> MVLGKVVGTVVASRKEPRIEGLSLLLVRACDPDGTPTGGAVVCADAVGAGVGEVVLYASGSSARQTEVTNNRPVDATIMAIVDLVEMGGDVRFRKD;>MADALGMIEVRGFVGMVEAADAMVKAAKVELIGYEK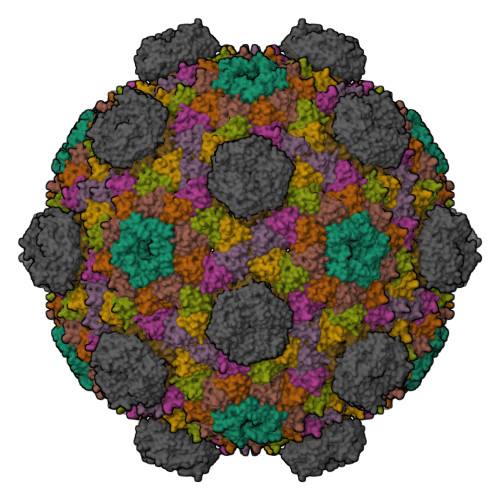TGGGYVTAVVRGDVAAVKAATEAGQRAAERVGEVVAVHVIPRPHVNVDAALPLGRTPGMDKSA[6x];>MSITLRTYIFLDALQPQLATFIGKTARGFLPVPGQASLWVEIAPGIAINRVTDAALKATKVQPAVQVVERAYGLLEVHHFDQGEVLAAGSTILDKLEVREEGRLKPQVMTHQIIRAVEAYQTQIINRNSQGMMILPGESLFILETQPAGYAVLAANEAEKAANVHLVNVTPYGAFGRLYLAGSEAEIDAAAEAAEAAIRSVSGVAQESFRDR[2x]>TSPSSPPAFRLETSDGGQDGAEVDKAQLGYGAGPPPMESRFQDEDRNFPPQIKVNLNYRKGAGASQPDLNRFDRDRLFNVVARGNPEDLAGLLEYLRRTSKYLTDSEYTEGSTGKTCLMKAVLNLQDGVNACIQPLLEIDRDSGNPQPLVNAQCTDEYYRGHSALHIAIEKRSLQCVKLLVENGANVHAKACGHFFQKNQDTCFYFGELPLSLAACTKQWDVVNYLLENPHQPASLQAQDSLGNTVLHALVMIADDSAENSALVVRMYDGLLQAGARLCPNVQLEGIPNLEGLTPLKLAAKEGKIEIFKHILQREFSAPCQSLSRKFTEWCYGPVRVSLYDLASVDSWEENSVLEIIAFHSRSPHRHRMVVLEPLNKLLQAKWDRLIPRFCFNFLCYLVYMLIFTAVAYHQPALEKQGFPPLKATAGNSMLLLGHILILLGGVYLLLGQLWYFWRRRLFIWISFMDSYFEILFLLQALLTVLSQVLCFLAIEWYLPLLVSSLVLGWLNLLYYTRGFQHTGIYSVMIQKVILRDLLRFLLVYLVFLFGFAVALVSLSREAQNSRTPAGPNATEVGQPGAGQEDEAPPYRSILDASLELFKFTIGMGELAFQEQLRFRGVVLLLLLAYVLLTYVLLLNMLIALMSETVNSVATDSWSIWKLQKAISVLEMENGYWWCRRKKQRAGVMLTVGTRPDGSPDERWCFRVGEMNWATWEQTLPRTLCEEPSGAAAPGVMKNPTPASQRGEDSASEEDHLPLQLLQSRDYKDDDDKAHHHHHH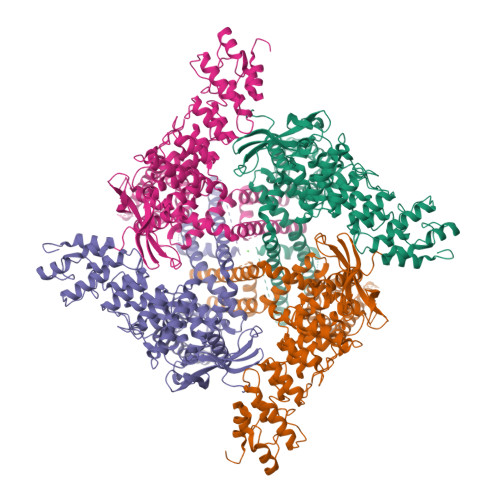[2x]> GEGDDAPGQSLYERLSQRM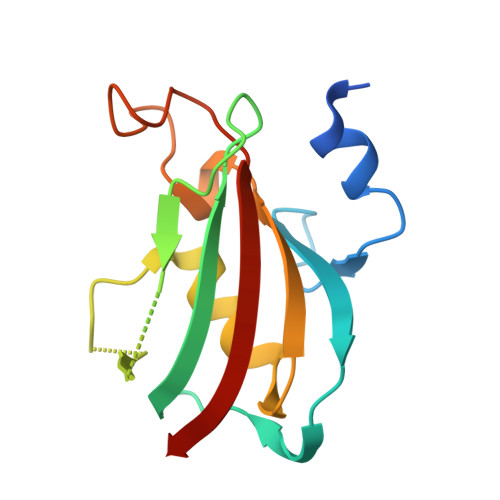LDISGDRGVLKDVIREGAGDLVAPDASVLVKYSGYLEHMDRPFDSNYFRKTPRLMKLGEDITLWGMELGLLSMRRGELARFLFKPNYAYGTLGCPPLIPPNTTVLFEIELLDFLD>[12x]MDVFVLDTSVFTNPEIYRTFEEDQRGAMETFIHLALNSRAEFYMPTSVYTEMRKIMDVGELWAEFEMVVKIRS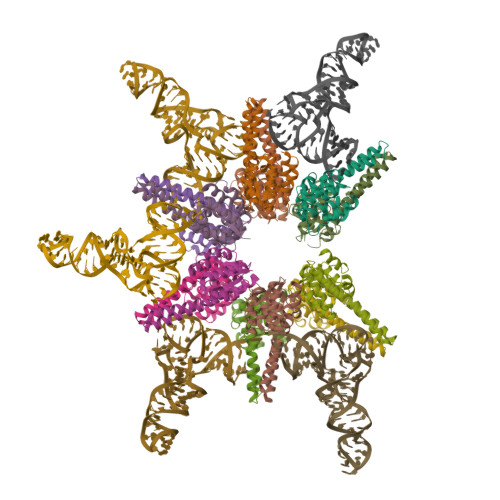PRRFQLTVPADFLYEFIEELRYRINKGLRIAEEHTREASGSEDVGKLIARLREKYREALRQGILDSKEDVDVLLLAYELDGVLVSADEGLRTWADKIGIKLIDPKNFKNILESLVRH> MKHHHHHHMKQNSPLDEENLTQENQDRGTHVDRGLASANVDFAFSLYKQLVLKAPDKNVIFSPLSISTALAFLSLGAHNTTLTEILKGLKFNLTETSEAEIHQSFQHLLRTLNQ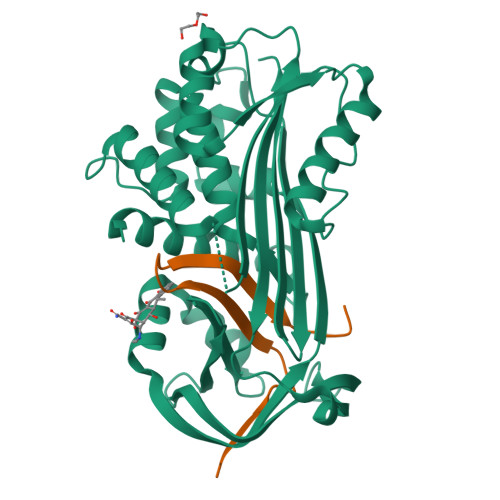SSDELQLSMGNAMFVKEQLSLLDRFTEDAKRLYGSEAFATDFQDSAAAKKLINDYVKNGTRGKITDLIKDLDSQTMMVLVNYIFFKAKFEMPFDPQDTHQSRFYLSKKKYVMVPMMSLHHLTIPYFRDEELSCTVVQLNYTGNASALFILPDQDKMEEVEAMLSQETLSRFFDSLEFREIGELYLPKFSISRDYNLNDILLQLGIEEAFTSKADLSGITGARNLAVSQVVHKAVLDVFEEGTEASAATALFIPLS;> LRMVETRTIVRFNRPFLMIIVDHFTWSIFFMSKVTNPKQA>TAPVPLDGTYRIEIQRSKQTYDYTPTPQPPDVNTWWAFRTSCTPTECLAAATMLDDNDHTQAKTPPVRPFLMQFGEGQWKSRPETVQFPCVGPNGSPSTQATTQLLALRPQPQGDLVGEMVVTVHSNECGQQGAVIRIPAVASRSG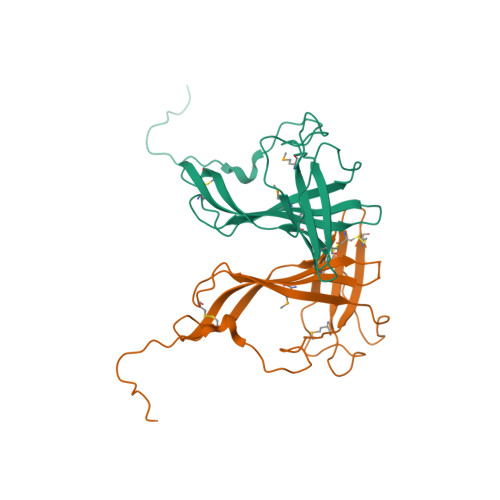DLPPAVTVPDPATIPDTPDTTSTATLTPPTTTAPGPGR[2x]>[2x]MGRGKRRAKTRNIAIASTKEVQWQGIFMIIVWLCVMGSLIFFANPEASRRVFAKFSHLQSFYGATSVAFAFATGLDILAYVNAVSDEKRVLSGILAYVDGVACISYLSMATLNLYFLVDSTQGNPVWLMRYAEWIITCPTLLYWCGLASRADRSSVSDIATADALLLAGGALSSILPSWPAFFVFAGSFATYIYVMLHMWGMFGKAMQPDFQPPPPLPRHALHLLRCEIVMSWSIFPLVEFLRRQGYIDFQVGEAMNCVADYAAKVGLAMIMVNCNLEQINALRVQQMHSALTGMLKVMRKTNLSSSRMAQLDGVDDDVKSWIMNEFSGSTDGKGGDDAKAQQRARGENLYFQ

Enzyme rhodopsins comprise the N-terminal rhodopsin domain and C-terminal enzyme domain, connected by a linker, and function as light-activated enzymes. Rh-PDE derived from Salpingoeca rosetta (SrRh-PDE) was first identified and exhibits light-dependent hydrolytic activity for both of cAMP and cGMP, whereas it lacks pump or channel activity. SrRh-PDE consists of the long N-terminal region, transmembrane domain (TMD), including the rhodopsin domain, C-terminal PDE domain, and 76-residue linker region connecting the TMD and PDE domain. Here, we present crystal structures of SrRh-PDE–TMD with and without the linker region, at 3.5 and 2.6 Å resolutions, respectively.

To obtain structural insight into the full-length Rh-PDE, we determined the 3.5 Å resolution crystal structure of Rh-PDE–TMD with the linker region (TMD–Linker, residues 33–378). The TMD–Linker structure superimposes well on the TMD structure (RMSD value of 0.84 Å over all Cα atoms). While the crystal packing is different between the TMD and TMD–Linker structures, both form a similar dimer interface. In one protomer, the C-terminal residues are observed up to Trp353. Residues 311 to 332 adopts a straight α-helix continuous from TM7, while residues 333–353 adopt a short loop and α-helix, turning back to the TMD. In the other protomer, the C-terminal residues are observed up to His320 and also adopt a straight α-helix. In the dimer, the α-helices in the linker regions cross each other, suggesting that the PDE dimer is swapped between the TMD dimer. Although the crystal packing might affect the conformation of the linker region, we can interpret its structure and connectivity with the TMD. In this model, TM7 is connected to the PDE domain via the linker regions crossing each other, resulting in the swapped position between the TMD and PDE domain.>[4x]NDLSGKTVIITGGARGLGAEAARQAVAAGARVVLADVLDEEGAATARELGDAARYQHLDVTIEEDWQRVVAYAREEFGSVDGLVNNAGISTGMFLETESVERFRKVVEINLTGVFIGMKTVIPAMKDAGGGSIVNISSAAGLMGLALTSSYGASK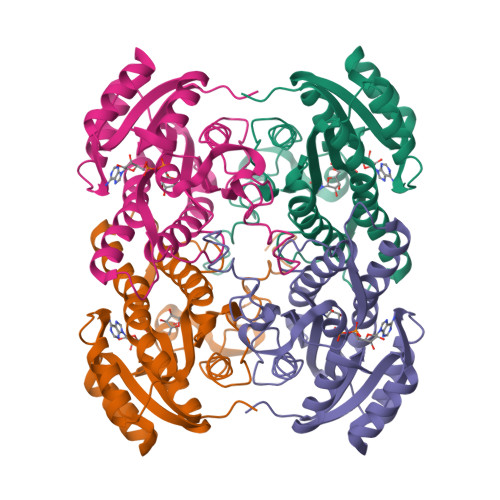WGVRGLSKLAAVELGTDRIRVNSVHPGMTYTPMTAETGIRQGEGNYPNTPMGRVGEPGEIAGAVVKLLSDTSSYVTGAELAVDGGWTTGPTVKYVMGQ>[4x]MGSSHHHHHHSSGENLYFQGHMTLSITSNFDAGAIDVVSCDSPDAIRLRVRGDNRSEFAQWFYYRLTGARGERCVMTFENAAECAYPSGWRNYSAVASYDRVDWFRVPTTFDGKTMTIDHTPEFDSIYYAYFEPYSEERHAAFLGAVQQLPQASVVELGRTVEGRPMSLLTLGTPETDGAPKKKVWIIARQHPGESMAEWFVEGLVKRLAGWGDWAGDPVARKLYDRVTFHIVPNMNPDGSVHGNLRTNAAGANLNREWMAPDAERSPEVLAVRDAIHAIGCDMFFDIHGDEDLPYVFVAGSEMLPSFTEQQGKEQTAFIEAFKVASPDFQTEHGYAASKYKEDALKLASKYIGHQFGCLSLTLEMPFKDNANLPDERVGWNGERSAALGAAMLAAILVHVDTFA

Carboxypeptidases (CPs) hydrolyse peptide bonds in target proteins to release C-terminal amino acids. One of the largest groups, carrying a single catalytic Zn2+ in the active site, is the M14 family. The C-terminal domain, which carries the Zn2+-containing active site, serves to classify this protein as a member of the M14D subfamily of carboxypeptidases. Although eukaryotic CCPs possess deglutamylase activity and are implicated in processing modified tubulin, the function and substrates of the bacterial family members remain unknown.

A potential cytosolic metallocarboxypeptidase from Burk­holderia cenocepacia has been crystallized and a synchrotron-radiation microfocus beamline allowed the acquisition of diffraction data to 1.9 Å resolution. BcCCP consists of 384 amino acids and forms a tetramer. BcCCP forms a tetramer arranged as a dimer of dimers. Residues Met1–Glu112 form the N-terminal domain, while the remaining 272 residues make up the CP domain. The N-terminal domain folds into a nine-stranded antiparallel β-sandwich. Here, the catalytic Zn2+ is coordinated by two histidines (His171 and His268), Glu174 in a chelating η2 interaction and a water molecule to give a pentacoordinated distorted tetrahedral geometry. The active-site cleft is occupied by an acetate derived from the crystallization conditions. This anion, which marks the binding site for the substrate carboxylate, is held in place by electrostatic interactions with Arg226, Asn235 and Arg236. The BcCCP structure displays an open configuration and the BmCCP structure a closed configuration with Tyr320 directed into the active site. Nearby, two differences, Gly253 and Asp256 in CP-A but Leu327 and Lys330 in BcCCP, make the the S1′ subsite much more shallow in the bacterial enzyme and replace an acidic residue with a basic one.>AVVTAGVAGLGAIDAASATQKTNRASTVKGGFDYDVVVVGGGFAGATAARECGLQGYRTLLLEARSRLGGRTFTSRFAGQEIEFGGAWVHWLQPHVWAEMQRYGLGVVEDPLTNLDKTLIMYNDGSVESISPDEFGKNIRIAFEKLCHDAWEVFPRPHEPMFTERARELDKSSVLDRIKTLGLSRLQQAQINSYMALYAGETTDKFGLPGVLKLFACGGWNYDAFMDTETHYRIQGGTIGLINAMLTDSGAEVRMSVPVTAVEQVNGGVKIKTDDDEIITAGVVVMTVPLNTYKHIGFTPALSKGKQRFIKEGQLSKGAKLYVHVKQNLGRVFAFADEQQPLNWVQTHDYSDELGTILSITIARKETIDVNDRDAVTREVQKMFPGVEVLGTAAYDWTADPFSLGAWAAYGVGQLSRLKDLQAAEGRILFAGAETSNGW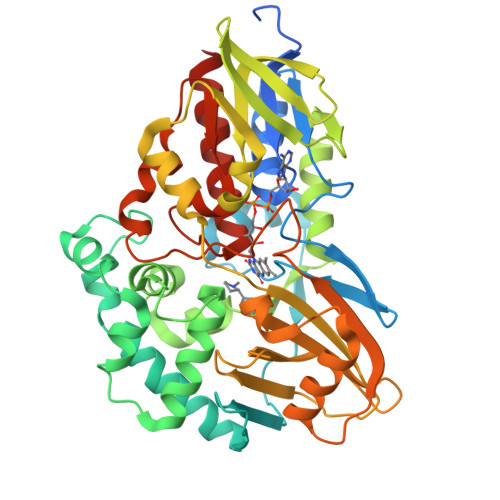HANIDGAVESGLRAGREVKQLLSLEHHHHHH[2x]>[8x]GTGVPETVFEELKRYVGWGD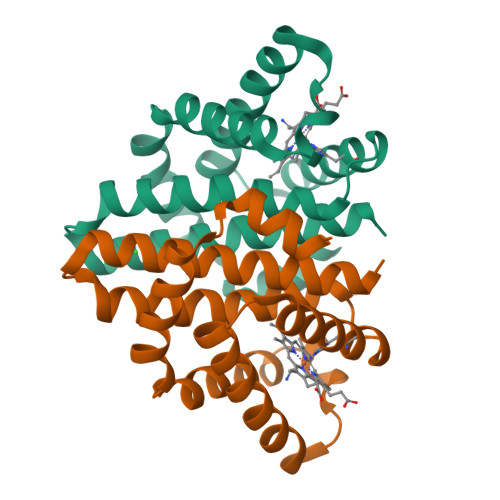GDERALRSLHGAAAPHFPRLAEEFYDRILGHEGARTALVGGESQVGHLKVTMIAWLDELLGGPWDEAYWDRRYRIGRVHVRIGLPQHYMFGAMNVHRTGLARLAYERFHGDPPELERVRNALGKVLDLELAVMLHTYREDL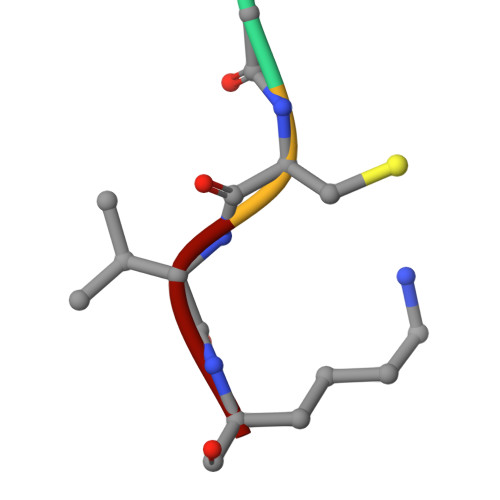> ACVK>MSDVSLKLSAKDIYEKDFEKTMARGYRREEVDAFLDDIIADYQKMADMNNEVVKLSEENHKLKKELEELR[2x];> NRLFRKR

In the Firmicutes phylum, GpsB is a membrane associated protein that coordinates peptidoglycan synthesis with cell growth and division. GpsB is a DivIVA-like protein that is highly conserved in Firmicutes. The full-length Sa GpsB is a relatively small protein of 114 residues. Its N-terminal domain homodimerizes as a coiled-coil, while its smaller C-terminal domain homotrimerizes, forming a hexamer as the biological unit. Dimerization of the N-terminal domain is facilitated by a pattern of nonpolar residues every three to four residues, promoting the formation of a hydrophobic core in the coiled-coil. This N-terminal domain is partitioned into three regions: a relatively short α-helix with approximately two turns (residues 10–16), a second longer α-helix (residues 28–70) that forms a coiled-coil, and an amphipathic 10-residue loop (residues 17–27) that links these two helices and intertwines with the adjacent protomer, ‘capping’ GpsB.

Remarkably, PBP4, the only class C PBP encoded in the S. aureus genome, which purportedly functions as both a carboxypeptidase and transpeptidase PBP, has a short, cytosolic C-terminal mini-domain with the sequence of N-R-L-F-R-K-R-K, satisfying the consensus GpsB-binding motif (S/T/N)-R-X-X-R-(R/K) found in S. aureus FtsZ and in orthologous PBPs found to bind to GpsB. To do so, we generated an R24A mutant because of its central role in the head-to-head interaction and its distance from the PBP-binding groove. This point mutation successfully disrupted the occluded crystal packing interface and allowed us to determine a 2.40 Å resolution structure of Sa PBP4 peptide bound to Sa GpsB. Unambiguous electron density for the Sa PBP4 C-terminal octapeptide, which adopted an α-helix, was resolved at the PBP-binding groove of GpsB. This structure clearly shows that two of these residues, Arg425 and Arg428, are key components of the Sa PBP4-Sa GpsB interaction, where they form multiple hydrogen bonds with the main chain amides of Sa GpsB Ile13, Tyr14, Lys16, and the sidechain hydroxyl of Tyr26. Furthermore, Arg425 and Arg428 form two salt bridges with the carboxyl sidechain of Asp32. Additionally, Sa GpsB Asp36 appears to play a major role in stabilizing the PBP4 α-helix by forming two hydrogen bonds with the backbone nitrogen of Arg425 and Leu426, an arrangement that is only possible when these two residues are part of an α-helix. Overall, the complex of Sa PBP4/Sa GpsB is very similar to Bs PBP1/Bs GpsB and is distinguished by the interactions of two Arg residues with the backbone and acidic sidechains lining the PBP-binding groove. A crystal structure of the Sa PBP4 C-terminal recognition sequence bound to the N-terminal domain of GpsB reveals a binding mode that mimics previously solved orthologous PBP/GpsB pairs. This discovery is notable because it was previously thought that only the N-terminal ‘mini-domain’ of transpeptidase PBPs (class A, class B) could bind to GpsB.>HHHHHHFNLPPGNYKKPKLLYCSNGGHFLRILPDGTVDGTRDRSDQHIQLQLSAESVGEVYIKSTETGQYLAMDTDGLVYGSQTPNEECLFLERLEENHYNTYISKKHAEKNWFLGLKKNGSCKRGPRTHYGQKAILFLPLP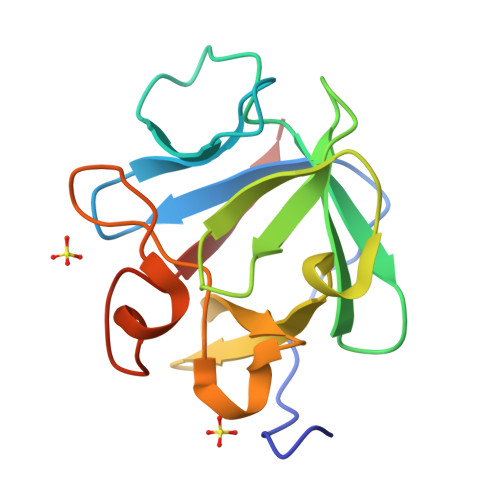VSSD[2x]> XQED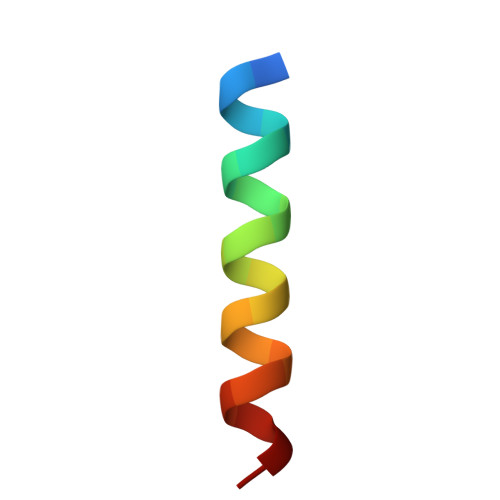IIRNIARHLAQVGDSMD The viral nucleoprotein (NP), a key component of the replication machinery, packages the viral genome into protective ribonucleoprotein particles. Although TiLV-NP is considerably smaller than its influenza counterpart and unrelated in sequence, it maintains the same topology and domain organisation. This comprises a head and body domain between which is a positively charged groove, where single-stranded RNA binds. In addition, an oligomerisation loop inserts into a hydrophobic pocket in the neighbouring NP, the flexible hinges of which allow variable orientation of adjacent NPs.

The RNA-bound TiLV-NP structure has been determined as part of distinct pseudo-symmetrical oligomers, including two tetrameric forms with pseudo-C2 and pseudo-C4 symmetries. The pseudo-C2 tetramer adopts an elongated structure, measuring 116 Å in length, 99 Å in width, and 70 Å in height. Within the pseudo-C2 tetramer, two A-form RNA double-stranded helices are inserted at the interfaces between opposite pairs of NP, whose single-stranded 5′ and 3′ extensions each bind one of the four NPs. The pseudo-C2 tetramer exhibits mean interface area of 1294 Å2 between NPs within one dimer and 994 Å2 at the dimer interface, while the pseudo-C4 tetramer exhibits a more uniform interface of 1313 Å2 between NPs. The accommodation of an A-form double-stranded RNA helix at the pseudo-C2 NP interface, as well as the oligomerisation into circular pentamers and hexamers, is facilitated by the flexible hinges of TiLV-NP (residues 288–293, 308–319). Within each of the positively charged grooves of TiLV-NPi and TiLV-NPi + 1, 8 nucleotides of RNA are bound as in the pseudo-C5 oligomers, but with free 5′ and 3′ ends, respectively. These two strands then come together at the NP-NP interface to form an A-form RNA double-helix comprising at least 10 base-pairs with a total of around 37 nucleotides visible. Two such structures bind to the pseudo-C2 oligomer. However, since the 40-mer vRNA loop used in the reconstitutions corresponds to 20 nucleotides from the 3′ and 5′ ends of one genome segment, the two observed RNA structures could each correspond to a single vRNA loop with a promoter-like fold, i.e. with a distal duplex (with the loop density missing), and single stranded terminii splayed out to bind in the two neighbouring NPs. In the pseudo-C2 structure, the duplex A-form RNA that splays out into single-stranded 3′ and 5′ extensions that bind to adjacent NPs, could also mimic the polymerase proximal promoter duplex separating into incoming and outgoing template strands, each binding an NP at the start of the RNP superhelix.

>MVRTTKTSMAAASTVAPEVAMDEGSPSTSQAQVELPRNLEVFNEACGHVFGSSFNREDNSVISDAAAFLFKMHTHSLDGQEAKVLRASEKKRERENAKKSRKAPEAGMRVGRSLILTSRWTEYCATCVPALGSKMKVIKASGDAAMIQMMKDHNSLLRVCVRIEVWKARYVSLVALDERIQTLEDAQWFPYLSGDSYRACPGLVGGYFAKKAAAGERGKNYKKLNQTAIIPPPRFLIIGHRLQIGDQVTLRELLASIAWGLCDGVLAECWSPSQGDGSIGVVVGLPLQATGSCFLVVASHGLSAIADSRIEGTGNTNLLEECIAIQKQDGVIKCKRSGKSLYHCLKETAGAVGR[4x]> GPAKQYDSVECPFCDEVSKYEKLAKIGQGTFGEVFKARHRKTGQKVALKKVLMENEKEGFPITALREIKILQLLKHENVVNLIEICRTKASPYNRCKGSIYLVFDFCEHDLAGLLSNVLVKFTLSEIKRVMQMLLNGLYY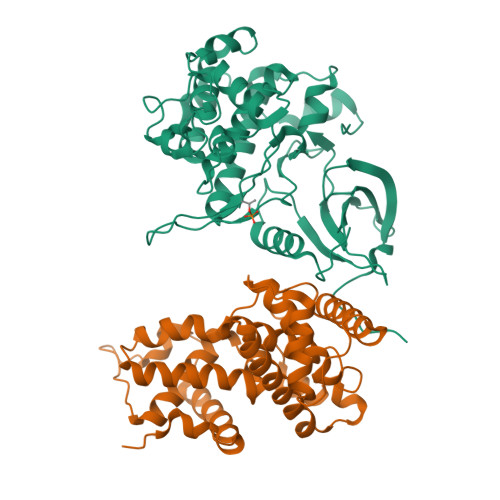IHRNKILHRDMKAANVLITRDGVLKLADFGLARAFSLAKNSQPNRYTNRVVTLWYRPPELLLGERDYGPPIDLWGAGCIMAEMWTRSPIMQGNTEQHQLALISQLCGSITPEVWPNVDNYELYEKLELVKGQKRKVKDRLKAYVRDPYALDLIDKLLVLDPAQRIDSDDALNHDFFWSDPMPSDLKGMLSTHLTSMFEYLAPPRRKGSQITQQSTNQSRNPATTNQTEFERVF;> GPEGERKNNNKRWYFTREQLENSPSRRFGVDPDKELSYRQQAANLLQDMGQRLNVSQLTINTAIVYMHRFYMIQSFTRFPGNSVAPAALFLAAKVEGQPKKLEHVIKVAHTCLHPQESLPDTRSEAYLQQVQDLVILESIILQTLGFELTIDHPHTHVVKCTQLVRASKDLAQTSYFMATNSLHLTTFSLQYTPPVVACVCIHLACKWSNWEIPVSTDGKHWWEYVDATVTLELLDELTHELLQILEKTPNRLKRIWNWR> WQPPWYAKEPVRIGSCKKQFSSF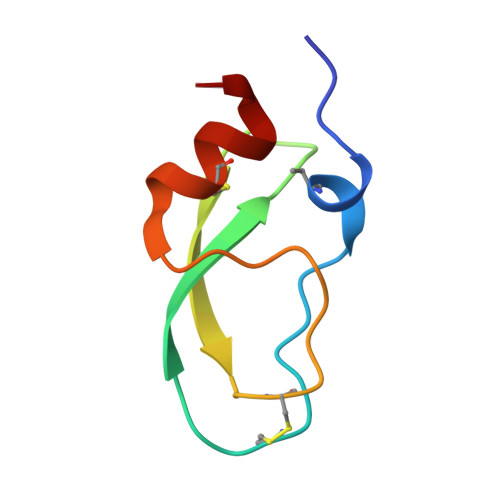YFKWTAKKCLPFLFSGCGGNANRFQTIGECRKKCLGK;> WQPPWYCKEPVRIGSCKKQFSSFYFKWTAKKCLPFLFSGCGGNANRFQTIGECRKKCLGK>KGLNYGSFTKEHVLLTPKGYREWV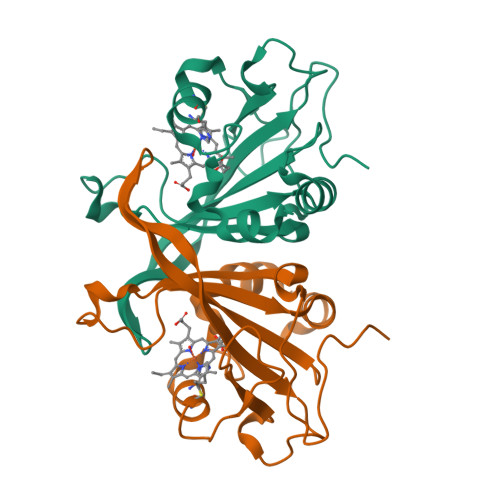FIGASVTPNELNDDKAAFPEFHNVYIDPTSWGHWKKTGEFRDGTVIVLELAGVGSKASPSGNGYFPGEFNGIEAMVKDSKRYPERPGNWAFFGFESYEAKQGIIQTDETCAACHKEHAAHDMVFTQFYPVLRAGKP[2x]(2R)-2-hydroxy-3,4-dioxopentyl 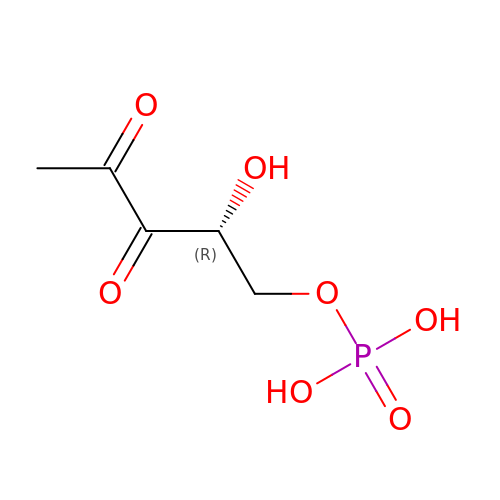dihydrogen phosphate | C5 H9 O7 P | DTZHMTDUIGHESZ-SCSAIBSYSA-N> AGFYVDGNTLYDANGQPFVMRGINHGHAWYKDTASTAIPAIAEQGANTIRIVLSDGGQWEKDDIDTIREVIELAEQNKMVAVVEVHDATGRDSRSDLNRAVDYWIEMKDALIGKEDTVIINIANEWYGSWDGSAWADGYIDVIPKLRDAGLTHTLMVDAAGW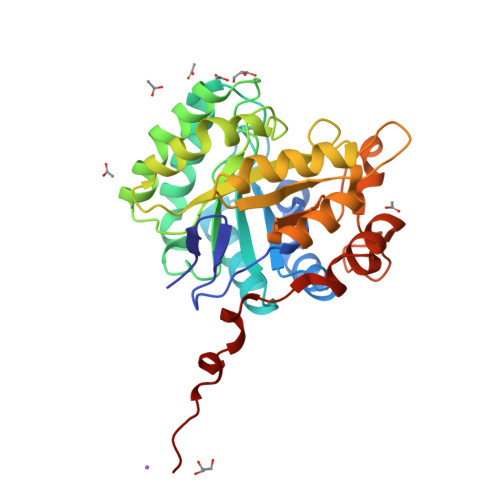GQYPQSIHDYGQDVFNADPLKNTMFSIHMYEYAGGDANTVRSNIDRVIDQDLALVIGEFGHRHTDGDVDEDTILSYSEETGTGWLAWSWKGNSTEWDYLDLSEDWAGQHLTDWGNRIVHGADGLQETSKPSTVFTDDNGGHPEPPT>[4x]MAHHHHHHMTKRIAVVTGGMGGLGEAVSIRLNDAGHRVVVTYSPNNTGADRWLTEMHAAGREFHAYPVDVADHDSCQQCIEKIVRDVGPVDILVNNAGITRDMTLRKLDKVNWDAVIRTNLDSVFNMTKPVCDGMVERGWGRIVNISSVNGSKGSVGQTNYAAAKAGMHGFTKSLALEIARKGVTVNTVSPGYLATKMVTAI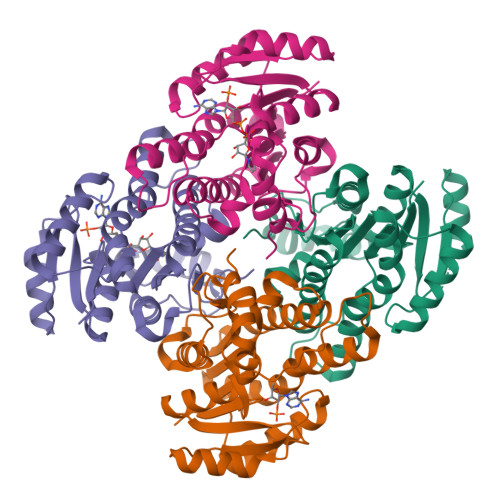PQDILDTKILPQIPAGRLGKPEEVAALVAYLCSEEAGFVTGSNIAINGGQHMH> GSHMQQWVDCEFTGRDFRDEDLSRLHTERAMFSECDFSGVNLAESQHR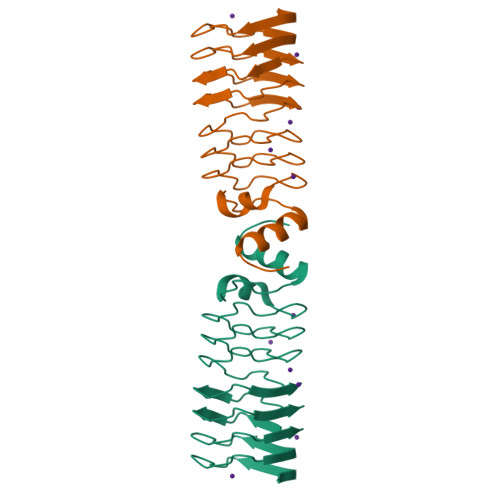GSAFRNCTFERTTLWHSTFAQCSMLGSVFVACRLRPLTLDDVDFTLAVLGGNDLRGLNLTGCRLRETSLVDTDLRKCVLRGADLSGARTTGARLDDADLRGATVDPVLWRTASLVGARVDVDQAVAFAAAHGLCLAGG(2S,5S,6S)-2,6-bis(azanyl)-5-oxidanyl-7-sulfooxy-heptanoic acid | C7 H16 N2 O7 S 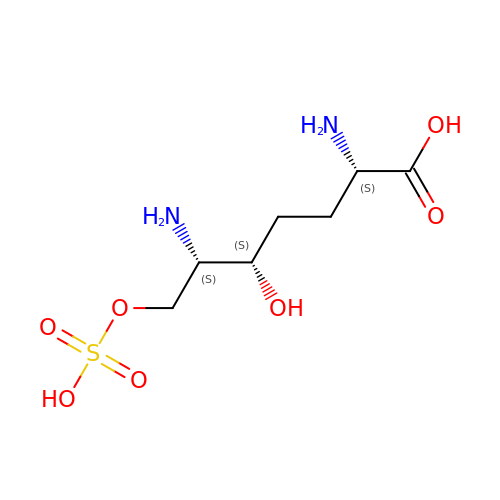| BPMKRAHMRLMOPA-ZLUOBGJFSA-N> MESVERKSESSYLGMRNMQPEQRLSLDPPRLRSTPQDELHDLLCVGFGPASLAIAIALHDALDPRLNKSASNIHAQPKICFLERQKQFAWHSGMLVPGSKMQISFIKDLATLRDPRSSFTFLNYLHQKGRLIHFTNLSTFLPARLEFEDYMRWCAQQFSDVVAYGEEVVEVIPGKSDPSSSVVDFFTVRSRNVETGEISARRTRKVVIAIGGTAKMPSGL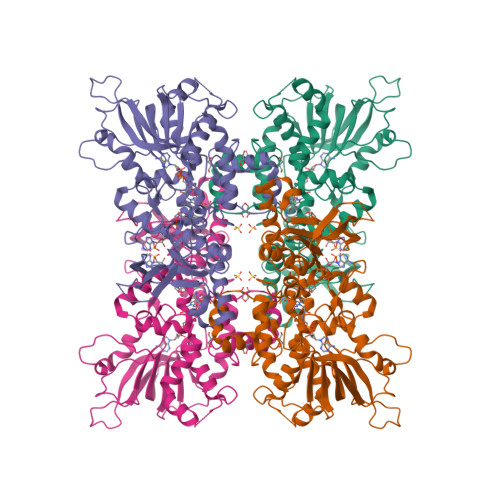PQDPRIIHSSKYCTTLPALLKDKSKPYNIAVLGSGQSAAEIFHDLQKRYPNSRTTLIMRDSAMRPSDDSPFVNEIFNPERVDKFYSQSAAERQRSLLADKATNYSVVRLELIEEIYNDMYLQRVKNPDETQWQHRILPERKITRVEHHGPQSRMRIHLKSSKPESEGAANDVKETLEVDALMVATGYNRNAHERLLSKVQHLRPTGQDQWKPHRDYRVEMDPSKVSSEAGIWLQGCNERTHGLSDSLLSVLAVRGGEMVQSIFGEQLERAAVQGHQLRAML> MNDDPTWYKDAIIYEVGVRCFFDSNNDGSGDIPGLTAKLDYIESLGVTAIWLLPFYASPLKDGGYDISDYRSLHPDFGTIEDFKVFLDEAHRRGIRVITELVLNHTSDQHQWFREARSNPNSPYRDYYVWSDTDDKYKDARIIFIDTERSNWTWDQEAGKYYWHRFFSHQPDLNYDNPKVQQEILDIVGYWLDMGVDGLRLDAVPYLYEREGTNCENLPETHEFLKKLRKFVDDNWPNRMLLAEANQWPEDVVAYFGNGDECHMAYHFPIMPRMYM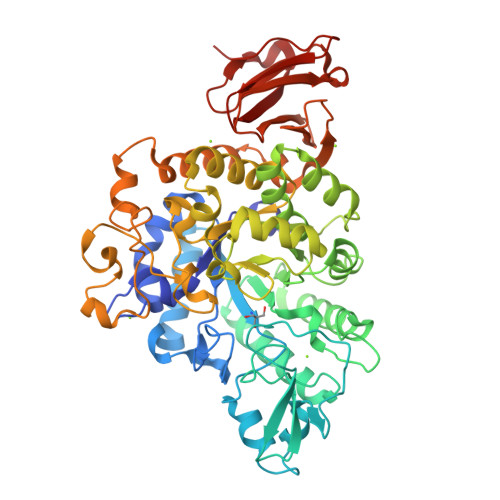ALRREDRHPITEILRRTPPIPETCQWALFLRNHDELTLEMVTDEERDYMYHEYAKDPRMRLNLGIRRRLAPLLDNSERRIQLMHLLLFTLPGTPIIYYGDEIGMGDNVYLGDRDGVRTPMQWSGDRNAGFSRANPQALYLPPIRDPVFTYEAVNVEAQEQVPTSLLNWMKRTIQIRKKYPVFGRGSIRFLQPSNRAVLAYIRQYQDTTILCACNLSRFCQAAELDLSDFKGLYPVELYGKTVFPQIGELPYLLTFGPHVFYWFELKPQEQLPH>[3x]GGLGPSDRQLLLFYLEQAEANLTTLTDAVDAFFTAVATNQPPKIFVAHSKFVILSAHKLVFIGDTLSRQAKAADVRSQVTHYSNLLSDL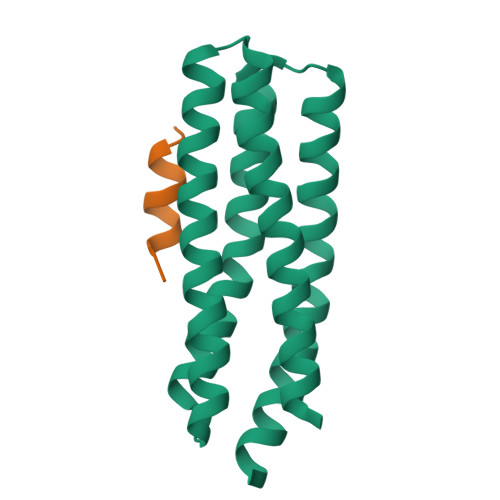LRGIVATTKAAALQYPSPSAAQDMVDRVKELGHSTQQFRRVLGQLAAA;>MDDLDALLADLESTTSHISK[3x]>[2x]LDLFVSPLGRVEGDLDVRVTINDGVVTSAWTEAAMFRGFEIILRGKDPQAGLIVCPRICGICGGSHLYKSAYALDTAWRTHMPPNATLIRNICQACETLQSIPRYFYALFAIDLTNKNYAKSKLYDEAVRRFAPYVGTSYQPGVVLSAKPVEVYAIFGGQWPHSSFMVPGGVMSAPTLSDVTRAIAILEHWNDNWLEKQWLGCSVDRWLENKTWNDVLAWVDENESQYNSDCGFFIRYCLDVGLDKYGQGVGNYLATGTYFEPSLYENPTIEGRNAALIGRSGVFADGRYFEFDQANVTEDVTHSFYEGNRPLHPFEGETIPVNPEDGRRQGKYSWAKSPRYAVPGLGNVPLETGPLARRMAASAPDAETHQDDDPLFADIYNAIGPSVMVRQLARMHEGPKYYKWVRQWLDDLELKESFYTKPVEYAEGKGFGSTEAARGALSDWIVIEDSKIKNYQVVTPTAWNIGPRDASEVLGPIEQALVGSPIVDAEDPVELGHVARSFDSCLVCTVH;>ASVLWFQGGACSGNTMSFLNADEPNVVDLIVDFGLDLLWHPSLGLELGNNAQKVFWDCAKGERPLDIFVFEGTVIEAPNGTGQMDMFAGRPMKDWVTDLAGAAQIVVAIGDCACFGGIPAMEPNPSGSTGLQFHKREKGGFLGPDFRSKMGLPVINVPGCPAHPDWITQILVALATGRAGDITLDDLHRPETFFKTFTQTGCTRVQFFEYKQSTLSFGEGTRTGCLFYEFGCRGPMTHSPCNRILWNRQSSKTRAGMPCLGCTEPEFPHFDLAPGTVFKTQKVSGMIPKEVPEGTDHLTYMGLAAAARIAAPQWSKEDMFVV[2x]

Here we determined the cryo-electron microscopy structure of the Mycobacterium smegmatis hydrogenase Huc and investigated its mechanism. Huc is a highly efficient oxygen-insensitive enzyme that couples oxidation of atmospheric H2 to the hydrogenation of the respiratory electron carrier menaquinone. Huc uses narrow hydrophobic gas channels to selectively bind atmospheric H2 at the expense of O2, and 3 [3Fe–4S] clusters modulate the properties of the enzyme so that atmospheric H2 oxidation is energetically feasible. The Huc catalytic subunits form an octameric 833 kDa complex around a membrane-associated stalk, which transports and reduces menaquinone 94 Å from the membrane.

Because of the flexibility exhibited by this complex, we performed 3D reconstruction of the individual Huc lobe from two datasets, obtaining resolutions of 1.52 Å and 1.67 Å. Density maps and the fourth coordinating residue of the 3 iron–sulfur clusters of HucS indicate they all have a [3Fe–4S] configuration. The redox properties of the Huc proximal and medial clusters may be further modified by an unusual d-isomer of histidine, indicated by the cryo-EM maps, at position 166 of HucL. In Huc, His166 also interacts with the proximal cluster, but the d-isomeric configuration shifts the position of the backbone carbonyl of His166 so that it interacts with a highly coordinated ligand in proximity to the medial cluster. We were unable to identify this ligand, although its elongated density suggests that it is not water, and it may have a role in tuning the redox potential of the medial [3Fe–4S] cluster. Although the narrow hydrophobic gas channels greatly kinetically favour H2 diffusion over O2, Fourier transform infrared (FTIR) spectroscopy analysis and the cryo-EM structure indicate that the active site of Huc isolated in ambient air is in an oxidized state with a bridging hydroxide ligand. The head group of menaquinone is stabilized by hydrogen bonding between its oxygen groups and the terminal hydroxyl of Tyr301 and the backbone carbonyl of Lys212, as well as π–π interactions with Tyr229 of HucS. Concordantly, analysis of the hydrophobic gas channels of Huc that provide H2 access to the active site indicates that they are markedly narrower than those of structurally characterized O2-sensitive and O2-tolerant [NiFe] hydrogenases.>[2x]MSVIEINDENFEEEVLKSDKPVLVDFWAPWCGPCRMIAPIIEE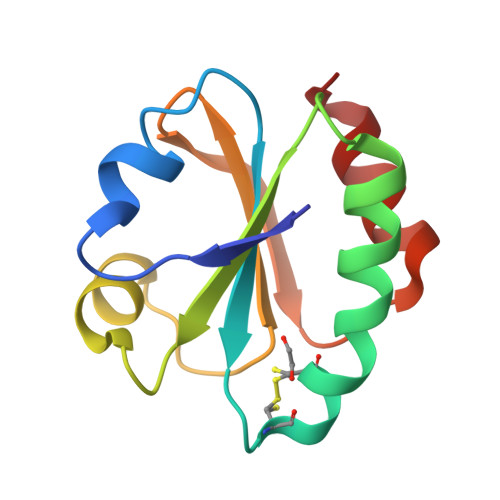LAEEYEGKVKFAKVNVDENPETAAKYGIMSIPTLLLFKNGEVVDKLVGARPKEALKERIEKHL> MKPTMAILERISKNSQENIDEVFTRLYRYLLRPDIYYVAYQNLYSNKGASTKGILDDTADGFSEEKIKKIIQSLKDGTYYPQPVRRMYIAKKNSKKMRPLGIPTFTDKLIQEAVRIILESIYEPVFEDVSHGFRPQ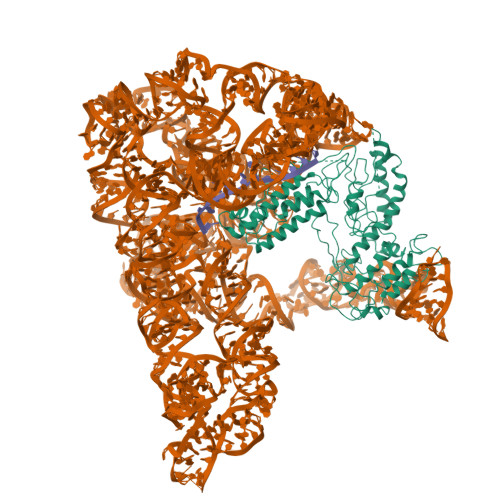RSCHTALKTIKREFGGARWFVEGDIKGCFDNIDHVTLIGLINLKIKDMKMSQLIYKFLKAGYLENWQYHKTYSGTPQGGILSPLLANIYLHELDKFVLQLKMKFDRESPERITPEYRELHNEIKRISHRLKKLEGEEKAKVLLEYQEKRKRLPTLPCTSQTNKVLKYVRYADDFIISVKGSKEDCQWIKEQLKLFIHNKLKMELSEEKTLITHSSQPARFLGYDIRVRRSGTIKRSGKVKKRTLNGSVELLIPLQDKIRQFIFDKKIAIQKKDSSWFPVHRKYLIRSTDLEIITIYNSELRGICNYYGLASNFNQLNYFAYLMEYSCLKTIASKHKGTLSKTISMFKDGSGSWGIPYEIKQGKQRRYFANFSECKSPYQFTDEISQAPVLYGYARNTLENRLKAKCCELCGTSDENTSYEIHHVNKVKNLKGKEKWEMAMIAKQRKTLVVCFHCHRHVIHKHK2-[3-[(1~{R})-1-[(2~{S})-1-[(2~{S})-2-cyclohexyl-2-thiophen-2-yl-ethanoyl]piperidin-2-yl]carbonyloxy-3-(3,4-dimethoxyphenyl)propyl]phenoxy]ethanoic acid | C37 H45 N O8 S | 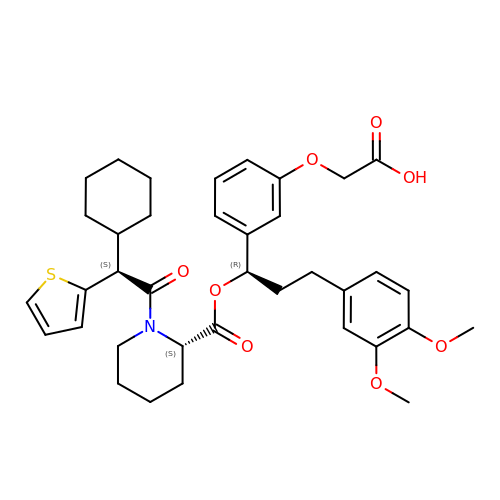YHWSKQSORLKYDT-CMKKOEAFSA-N> SRPLSDQEKRKQISVRGLAGVENVTELKKNFNRHLHFTLVKDRNVATPRDYYFALAHTVRDHLVGRWIRTQQHYYEKDPKRIYYLSLEFYMGRTLQNTMVNLALENACDEATYQLGLDMEELEEIEEDAGLGNGGLGRLAACFLDSMATLGLAAYGYGIRYEFGIFNQKICGGWQMEEADDWLRYGNPWEKARPEFTLPVHFYGRVEHTSQGAKWVDTQVVLAMPYDTPVPGYRNNVVNTMR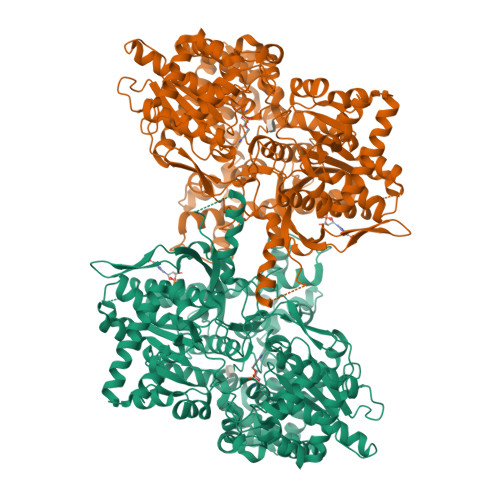LWSAKAPNDFNLKDFNVGGYIQAVLDRNLAENISRVLYPNDNFFEGKELRLKQEYFVVAATLQDIIRRFKSSKFGCRDPVRTNFDAFPDKVAIQLNDTHPSLAIPELMRVLVDLERLDWDKAWEVTVKTCAYTNHTVIPEALERWPVHLLETLLPRHLQIIYEINQRFLNRVAAAFPGDVDRLRRMSLVEEGAVKRINMAHLCIAGSHAVNGVARIHSEILKKTIFKDFYELEPHKFQNKTNGITPRRWLVLCNPGLAEIIAERIGEEYISDLDQLRKLLSYVDDEAFIRDVAKVKQENKLKFAAYLEREYKVHINPNSLFDVQVKRIHEYKRQLLNCLHVITLYNRIKKEPNKFVVPRTVMIGGKAAPGYHMAKMIIKLITAIGDVVNHDPVVGDRLRVIFLENYRVSLAEKVIPAADLSEQISTAGTEASGTGNMKFMLNGALTIGTMDGANVEMAEEAGEENFFIFGMRVEDVDRLDQRGYNAQEYYDRIPELRQIIEQLSSGFFSPKQPDLFKDIVNMLMHHDRFKVFADYEEYVKCQERVSALYKNPREWTRMVIRNIATSGKFSSDRTIAQYAREIWGVEPSRQRLPAPDEKIP> GSGNASSGALGTTGGAT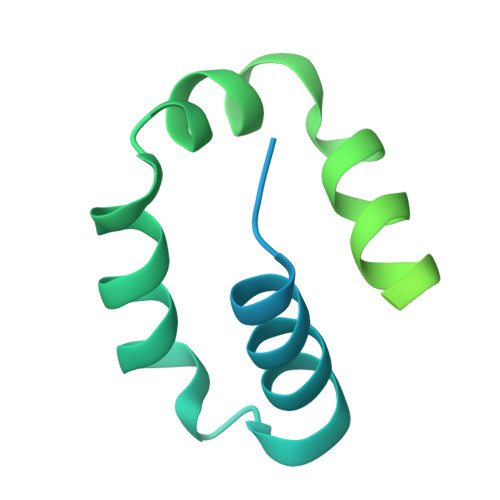DAAQGGPPGSIGLTVEDLLSLRQVVSGNPEALAPLLENISARYPQLREHIMANPEVFVSMLLEAVGDNMQDVMEGADDMVEGEDIEVTGEAAAAGLGQGEGEGSFQVDYTPEDDQAISRLCELGFERDLVIQVYFACDKNEEAAANILFSDHAD> MSSMNFNPFQNWFEKPPNPVPSINFVSLADSFFPKSQSPNFASIGLPKFSKKSP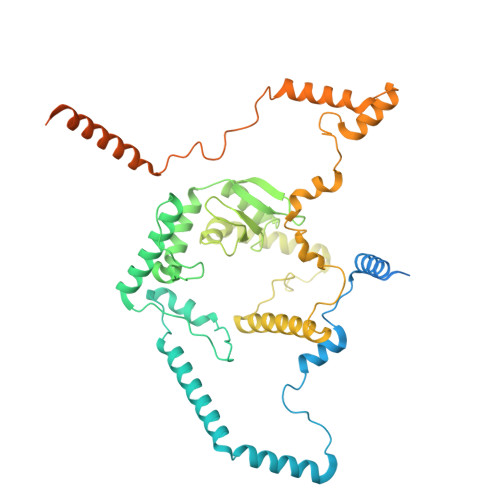KPETAGTDEPGPYKQIAEQFLWECENIPDYRHTPEVDKLLNEDPVFEKKENPSTEEIEAEQKWWESFRASPVVQFMTRAEEIADDMNKMELEDNDTPYRKEDKDYWRAIPHVPGFDGRPMPRKAIKSKEESDDKFWDFMKQFLFGLWGFRQRPYPPGRPIDVAQAIGYKRLEKRYYDFIMKTGGWWYKDRLGRSRGPCEIITLKTAYGAGIIDRDTFIWGEDMDEWAPIHMVYGLEPAIATWEVRLGAAATAFLHKLQKGIPPWVPLKGREPKTYKQLQKEAIESKKRDMAVLEANGGVWPGVRTPSHALFLWASGSELTTVLESDHMPNKFIPKQLRLELAKVIPGLRPWEVISIEQAMDQISYGGEWYREPLGTYTTGPPYIREWNRSVMRLFRIFYNLSVRVGQKLERTVPGFDTIMDKVQKDYDKRIARRMKRREEELREEDLKHYSGRTDEDEEEEEEEDDDSNSKKD>[6x]MPDMKLFAGNATPEL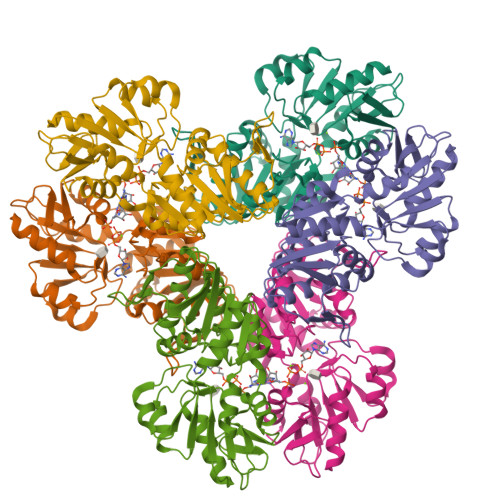AQRIANRLYTSLGDAAVGRFSDGEVSVQINENVRGGDIFIIQSTCAPTNDNLMELVVMVDALRRASAGRITAVIPYFGYARQDRRVRSARVPITAKVVADFLSSVGVDRVLTVDLHAEQIQGFFDVPVDNVFGSPILLEDMLQLNLDNPIVVSPDIGGVVRARAIAKLLNDTDMAIIDKRRPRANVSQVMHIIGDVAGRDCVLVDDMIDTGGTLCKAAEALKERGAKRVFAYATHPIFSGNAANNLRNSVIDEVVVCDTIPLSDEIKSLPNVRTLTLSGMLAEAIRRISNEESISAMFEHHHHHHH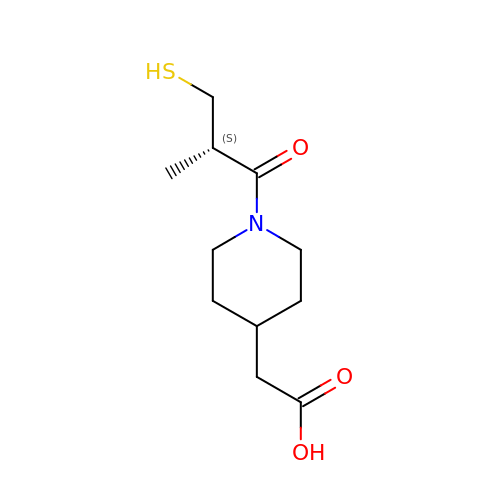2-[1-[(2S)-2-methyl-3-sulfanyl-propanoyl]piperidin-4-yl]ethanoic acid | C11 H19 N O3 S | FPXOJLHTOWZYDD-MRVPVSSYSA-N> GPLGSPEFDNNIENIGDGAEVVKRTEDTSSDKWGVTQNIQFDFVKDKKYNKDALILKMQGFINSKTTYYNYKNTDHIKAMRWPFQYNIGLKTNDPNVDLINYLPKNKIDSVNVSQTLGYNIGGNFNSGPSTGGNGSFNYSKTISYNQQNYISEVEHQNSKSVQWGIKANSFITSLGKMSGHDPNLFVGYKPASQNPRDYFVPDNELPPLVHSGFNPSFIATVSHEKGSGDTSEFEITYGRNMDVTHATRRTTHYGNSYLEGSRIHNAFVNRNYTVKYEVNWKTHEIKVKGHN

With the exception of α-hemolysin, which is homo-heptameric, leukotoxins are bipartite toxins, formed by the non-covalent association of two distinct proteins, a class S and a class F component of approximately 31 and 34 kDa, respectively, into a likely octameric species. Panton-Valentine leukocidin (PVL) is associated with necrotizing skin infections, such as boils, and plays an important role in the poor prognosis of necrotizing pneumonia. Two additional structural domains are also found: the rim domain anchors the protein to the membrane surface, while the stem domain, closely apposed to the core β-sandwich in the soluble form, contributes two β-strands to the pore β-barrel. Since the binding of LukS-PV to the membrane is a saturable process, the necessary presence of a LukS-PV receptor on the cell surface was thus proposed. This was recently confirmed by Spaan et al. who showed that the C5a receptor is required for the binding of LukS-PV to human neutrophils.

The mutants exhibiting significantly decreased binding abilities with respect to wild-type LukS-PV were: R73A, Y184A, T244A, H245A, and Y250A, with Ki values ranging from 1.8 to 6.2 nM, i.e. a 69- to 238-fold increase compared to the Ki value of wild-type LukS-PV. Four LukS-PV mutants (R73A, Y184A, T244A, and Y250) displayed significant alterations for all measured parameters, i.e. at least 50-fold decrease in affinity for hPMN membranes, 2-fold decrease in the slope of Ca2+ influx and 2- to 10-fold reduction in pore-forming capacity. Crystals of the Y184A mutant were obtained at a lower pH 6.50, but the conditions were otherwise identical. The latter belonged to the P41212 space group with cell parameters a = 104.86 Å and c = 106.87 Å, 1 molecule per asymmetric unit, and diffracted up to 2.33 Å. In the case of the rim domain, wild-type LukS-PV and mutants T244A, Y246A and N248A displayed only small differences, with r.m.s. deviations comprised between 0.20 Å and 0.30 Å, whereas the structure of the rim domain of the Y184A and Y250A mutants were markedly different, with r.m.s. deviations of 1.10 Å and 1.28 Å, respectively, when compared to the wild-type LukS-PV structure. Other significant variations in the conformation of the rim domain were only found in the structure of the Y184A mutant, where residues V179–Q186 were affected, as well as in the conformation of the Y250A mutant, where two loops (V179–Q186 and R241–A250) showed structural variations. As the result of the Y184A mutation, the hydrogen bond found in the wild-type LukS-PV structure between Y184OH and S249OG was lost, and the loop was reorganized with a displacement of 6.0 Å for the CA atom at position 184. For both Y184A and Y250A mutants, crystallization was achieved in different conditions than those for wild-type LukS-PV and the other mutants, resulting in a different crystal packing.> MQLRKLLLPGLLSVTLLSGCAMGATQGTADKDAQITQDWSVEKLYAEAQDELNSSNYTRAVKLYE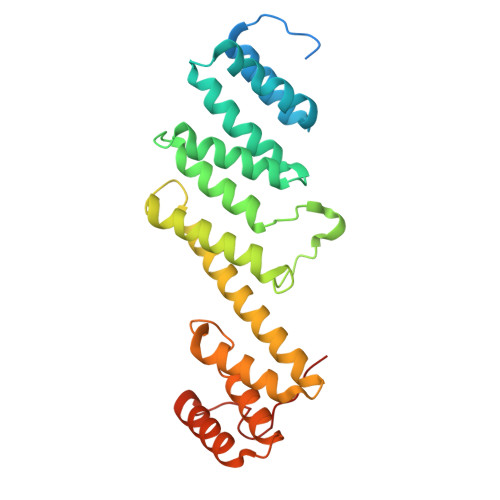ILESRFPTSRHARQSQLDTAYAYYKDDEKDKALAAIERFRRLHPQHPNMDYALYLRGLVLFNEDQSFLNKLASQDWSDRDPKANREAYQAFAELVQRFPNSKYAADATARMVKLVDALGGNEMSVARYYMKRGAYIAAANRAKKIIGSYQNTRYVEESLAILELAYKKLDKPQLAADTRRVLETNFPKSPFLTHAWQPDDMPWWRYWH> SASPA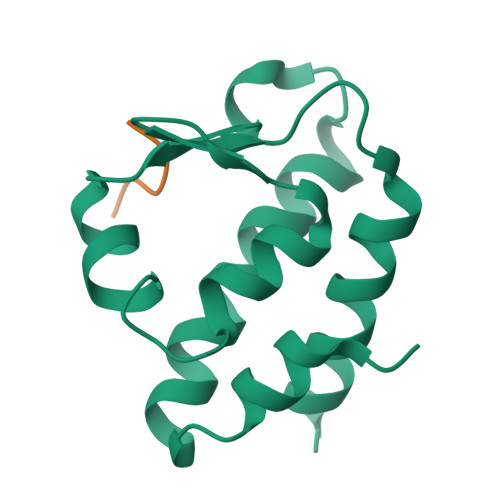VAELCQNTPETFLEASKLLLTYADNILRNPSDEKYRSIRIGNTAFSTRLLPVRGAVECLFEMGFEEGETHLIFPKKASVEQLQKIRDLIAIERSS;> DDLYG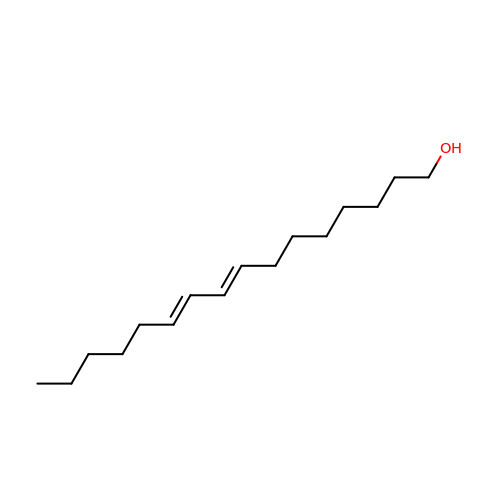(8E,10Z)-HEXADECA-8,10-DIEN-1-OL | C16 H30 O | IUVFLMAKSXSTQK-NMMTYZSQSA-N>STTKCTVSHEVADCSHLKLTQVPDDLPTNITVLNLTHNQLRRLPAANFTRYSQLTSLDVGFNTISKLEPELCQKLPMLKVLNLQHNELSQLSDKTFAFCTNLTELHLMSNSIQKIKNNPFVKQKNLITLDLSHNGLSSTKLGTQVQLENLQELLLSNNKIQALKSEELDIFANSSLKKLELSSNQIKEFSPGCFHAIGRLFGLFLNNVQLGPSLTEKLCLELANTSIRNLSLSNSQLSTTSNTTFLGLKWTNLTMLDLSYNNLNVVGNDSFAWLPQLEYFFLEYNNIQHLFSHSLHGLFNVRYLNLKRSFTKQSISLASLPKIDDFSFQWLKCLEHLNMEDNDIPGIKSNMFTGLINLKYLSLSNSFTSLRTLTNETFVSLAHSPLHILNLTKNKISKIESDAFSWLGHLEVLDLGLNEIGQELTGQEWRGLENIFEIYLSYNKYLQLTRNSFALVPSLQRLMLRRVALKNVDSSPSPFQPLRNLTILDLSNNNIANINDDMLEGLEKLEILDLQHNNLARLWKHANPGGPIYFLKGLSHLHILNLESNGFDEIPVEVFKDLFELKIIDLGLNNLNTLPASVFNNQVSLKSLNLQKNLITSVEKKVFGPAFRNLTELDMRFNPFDCTCESIAWFVNWINETHTNIPELSSHYLCNTPPHYHGFPVRLFDTSSCKDSAPFELFFMINTSILLIFIFIVLLIHFEGWRISFYWNVSVHRVLGFKEIDRQTEQFEYAAYIIHAYKDKDWVWEHFSSMEKEDQSLKFCLEERDFEAGVFELEAIVNSIKRSRKIIFVITHHLLKDPLCKRFKV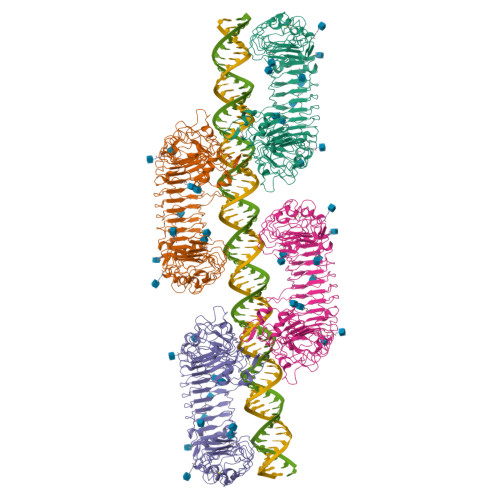HHAVQQAIEQNLDSIILVFLEEIPDYKLNHALCLRRGMFKSHCILNWPVQKERIGAFRHKLQVALGSKNSVHSNSLEVLFQ[4x]>AEPFAKLEQDFGGSIGVYAMDTGSGATVSYRAEERFPLCXSFKGFLAAAVLARSQQQAGLLDTPIRYGKNALVPWSPISEKYLTTGMTVAELSAAAVQYSDNAAANLLLKELGGPAGLTAFMRSIGDTTFRLDRWELELNSAIPSDARDTSSPRAVTESL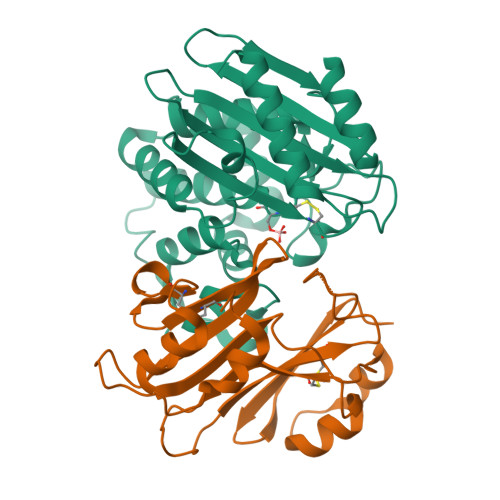QKLTLGSALAAPQRQQFVDWLKGNTTGNHRIRAAVPADWAVGDKTGTCGVYGTANDYAVVWPTGRAPIVLAVYTRAPNKDDKHSEAVIAAAARLALEGLGVNGQ[2x];>AGVMTGAKFTQIQFGMTRQQVLDIAGAENCETGGSFGDSIHCRGHAAGDYYAYATFGFTSAAADAKVDSKSQEKLLAPSAPTLTLAKFNQVTVGMTRAQVLATVGQGSCTTWSEYYPAYPSTAGVTLSLSCFDVDGYSSTGFYRGSAHLWFTDGVLQGKRQWDLV[2x]>AMGKCPTKVVLLRNMVGAGEVDEDLEVETKEECEKYGKVGKCVIFEIPGAPDDEAVRIFLEFERVESAIKAVVDLNGRYFGGRVVKACFYNLDKFRVLDLAEQ[2x];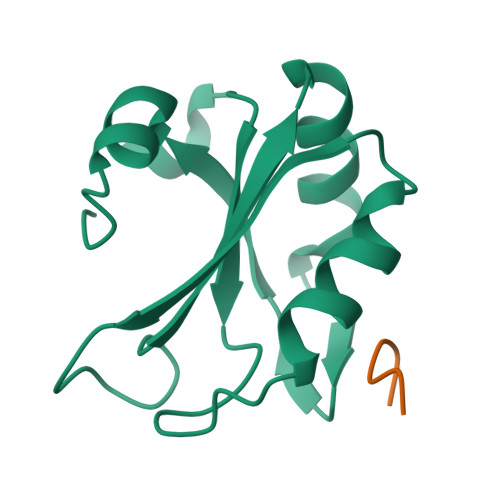>[2x]KSRWDE> MVANPEHYIKHPLQNRW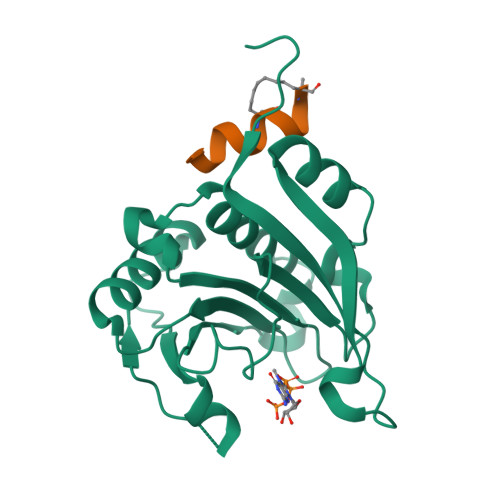ALWFFKNDKSKTWQANLRLISKFDTVEDFWALYNHIQLSSNLMPGCDYSLFKDGIEPMWEDEKNKRGGRWLITLNKQQRRSDLDRFWLETLLCLIGESFDDYSDDVCGAVVNVRAKGDKIAIWTTECENREAVTHIGRVYKERLGLPPKIVIGYQSHADTATKSGSTTKNRFVV;> XKKRYSREQLLLFQRLX>PMAAHEASSLYSEEKAKLLREMMAKIEDKNEVLDQFMDSMQLDPETVDNLDAYSHIPPQLMEKCAALSVRP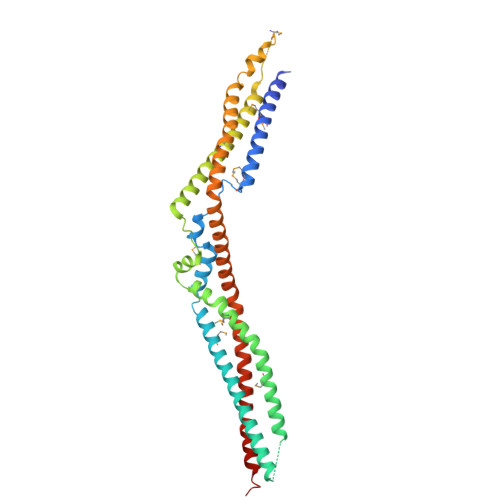DTVRNLVQSMQVLSGVFTDVEASLKDIRDLLEEDELLEQKFQEAVGQAGAISITSKAELAEVRREWAKYMEVHEKASFTNSELHRAMNLHVGNLRLLSGPLDQVRAALPTPALSPEDKAVLQNLKRILAKVQEMRDQRVSLEQQLRELIQKDDITASLVTTDHSEMKKLFEEQLKKYDQLKVYLEQNLAAQDRVLCALTEANVQYAAVRRVLSDLDQKWNSTLQTLVASYEAYEDLMKKSQEGRDFYADLESKVAALLERTQSTCQAREAARQQLLDRELK[2x]The Prx subfamily enzyme Prx1, also typically called 2-Cys Prx, is among the most highly expressed, soluble proteins in the cell, and is characterized by two conserved cysteine residues. We used the mechanistically well understood E. coli as a prototype to construct a chimeric Prx, EcAhpC1-186-YFSKHN, composed of EcAhpC (residues 1–186) and the C-terminal YFSKHN-segment of human Prx 2, to be compared with wild-type (WT) EcAhpC. The chimeric EcAhpC1-186-YFSKHN described here demonstrates, that transformation of the human C-terminal YFSKHN-helix into the related bacterial AhpC confers sensitivity to over-oxidation on the chimeric enzyme. Structural details of the oxidized and reduced chimeric EcAhpC1-186-YFSKHN provide novel insights into sub-steps during the catalysis of peroxide reduction, enabling the transition from a fully folded to a locally unfolded conformation. Together with mutational and enzymatic studies these data unravel the fundamental role of the C-terminal tail as a molecular switch that mediates the structural transition between the FF and LU state during the catalytic cycle.

To shine a light on the redox modulated structural alterations in the active site, the crystallographic structure of reduced EcAhpC1-186-YFSKHN was determined to 3.1 Å resolution. No disulphide bond between CP47 and CR166′ was observed in any of the active site interfaces of the decameric EcAhpC1-186-YFSKHN, confirming that the structure fairly represents the reduced form of EcAhpC1-186-YFSKHN. Except for the C-terminus, clear electron density was observed for all the residues and the resolving cysteine (chains C, E, F, H and J), which is located about 10 Å away from the peroxidatic one. Interestingly, two different active site conformations were observed in the reduced EcAhpC1-186-YFSKHN structure, where the residues in the active site region are clearly defined in the electron density map except for the side chains of F45 and V46. The first conformation (chains B-J) reveals that the peroxidatic CP47 adopts helical conformation, bringing the CP47 in a narrow solvent accessible pocket, which is surrounded by the highly conserved active site residues P40, T44 and R120. In the second active site conformation (chain A), the first turn of α2-helix is partially unfolded to place CP47 in the loop conformation. While in the second active site of reduced EcAhpC1-186-YFSKHN, the unfolded CP47 adopts a lower magnitude of rotation, thereby preventing its full exposure towards CR166′ to form a disulphide. For clarity, we termed the first and second active sites of the reduced EcAhpC1-186-YFSKHN as FFlike and LUlike, respectively, to denote the folded and unfolded CP47 in the active site environments. Because of the magnitude of displacement, the data indicate that the FFlike and LUlike state, adopt intermediate conformations, lying between the catalytic FF and LU conformation.

>MSLINTKIKPFKNQAFKNGEFIEITEKDTEGRWSVFFFYPADFTFVCPTELGDVADHYEELQKLGVDVYAVSTDTHFTHKAWHSSSETIAKIKYAMIGDPTGALTRNFDNMREDEGLADRATFVVDPQGIIQAIEVTAEGIGRDASDLLRKIKAAQYVASHPGEVCPAKWKEGEATLAPSLDLVGKYFSKHN[10x]>LLQEEEEGLPLVGRVAAGEPLPAQWHIEGHYQVDPSLFKPNADFLLRVSGMSMKDIGIMDGDLLAVHKTQDVRNGQVVVARIDDAVTVARLKKQGNKVELLPENSEFKPIVVDLRQQSFTIEGLAVGVIRNGD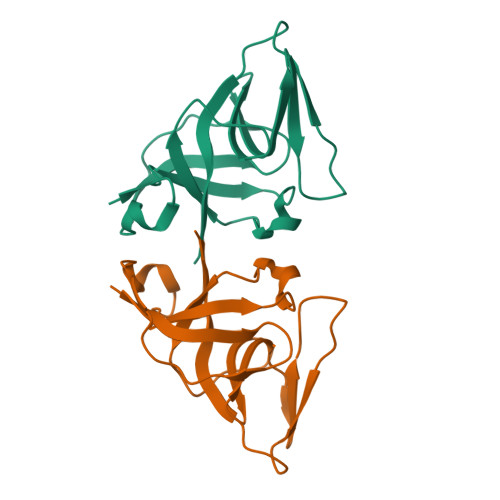WL[2x]> MANYNYIVDTGVIVADTADVLSDVEAEFRAAL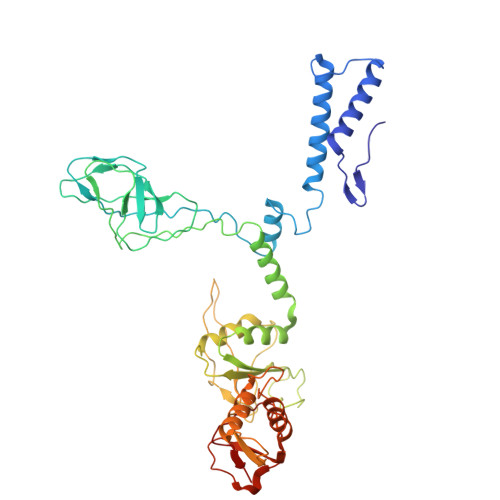GANINLAASTPQGSLVAAEAIARSSVMRNEARIANTINPNVSFGTFLDAICALMGIERGSDLSTFGYGVQVTGRSQTRISTGSRVQTPAGAIFTVMSDVTIPAGGVATIDIKSQEYGNIPLPVGNLIIIDGTIGWSGAKVIASTRVDPGSRQMSDAELKNARVNRLAIQGRNSTMAIKAYVSAVPNVTSVNVIENNTGAVQVVNGVSFTLPYAVWVCVAGNPDKQAVADALWAAHNGGTPWDYGATNNGVPVDGPNGVPVRDPASGRKYVVKWTTPIMYDGYVNVTVQQGSSSVAPEAIQNAVVNYAQGKVEGEEGLVVGASLSAFEVAGAIAREIPGIYIKLCQVACVAAGSPAPAPGDFTSEYVMSAFGQATISVGNVRVTFV N-ethyl-4-{[4-(1H-indol-3-yl)-5-iodopyrimidin-2-yl]amino}piperidine-1-carboxamide 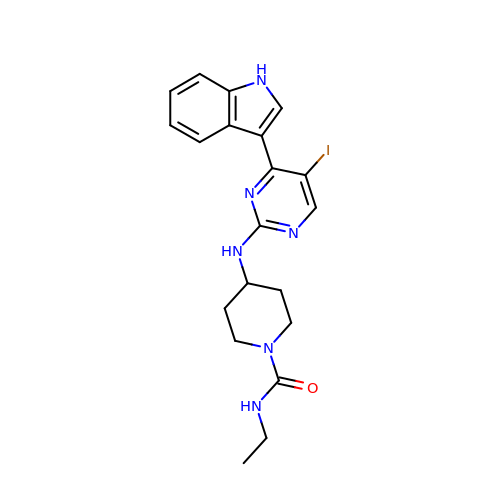| C20 H23 I N6 O | AUFRUDIABNXVLI-UHFFFAOYSA-N>GSMAETKAKAEDLKMQGNKAMANKDYELAINKYTEAIKVLPTNAIYYANRAAAHSSLKEYDQAVKDAESAISIDPSYFRGYSRLGFAKYAQGKPEEALEAYKKVLDIEGDNATEAMKRDYESAKKKVEQSLNL[2x];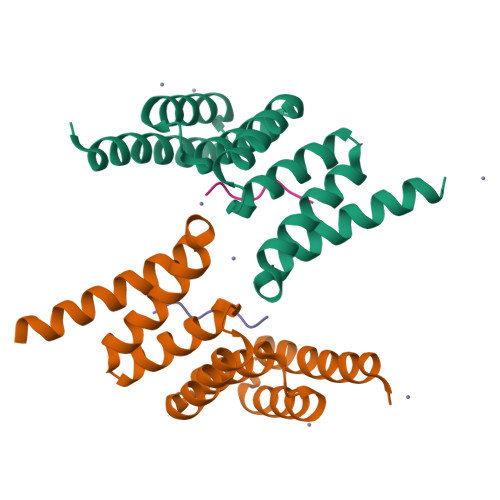>[2x]PTVEEVD>[12x]EEIMRDDNMMFITKKMIEIRNLLQKVGQGSTVTLPSIVVIGSQSSGKSSVLEAIVGHEFLPKGSNMITRRPIELTLVNDPEAKVDYGEFPDLGLARVTDFSLIQKTLTELNQSVPESECVTDDPIRLTIHSPNIPDLSLIDLPGYIQVAGENQPRELKRKITELCDKYIRGPNIILAISAADTDLANSTALQASRRVDPRGERTIGVITKMDLVEPEKGAAILSDRQYPLKLGYVGVISKLPPQSGLFRRDTGNLLASINRNEKNYFGSHPTEFGPDSGVSTGVMTLRKKLLQVLEQQMSSKLNETTEAIQRELEETT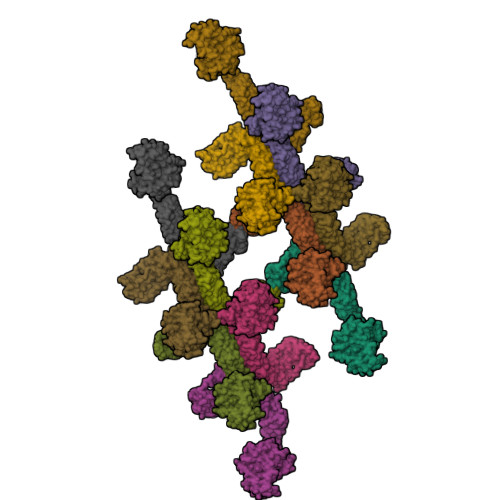YQFKVQYNEQPMSAESYLAASLDDFKHQFHEFASSFGRPQLQTLLKDALDQKVLDQLAARYWNRPIEDLSPAPREPDNIIDLPKADPDSPYWHRQLDTACSGLTRLGVGRLAATVAASAIQQHVEKLLDKSSFAKHPSARKVISDAAATVLADRSYATSDGIEISLKPYKFDPDIQPNEWAQGREHVVGVLQAELEQCQAAMKALENSVGGRKKLKEVMSFVDKARKGEIIVEGDHPSGAGGFSAALLARGREAVFLRDRADILSLRIQAAKSRQCKTLTNKYYCPEVFLDAVATKLAQTAVLFLNVEMLNDFYVRFPREVEAKLHEHMHAGGGLEKFAREDPKVRRHLDLIRRKELLETVLGKIEELHRISSGTAG>SYRSRSAFKLLEVNERHQILRPGLRVLDCGAAPGAWSQVAVQKVNAAGTDPSSPVGFVLGVDLLHIFPLEGATFLCPADVTDPRTSQRILEVLPGRRADVILSDMAPNATGFRDLDHDRLISLCLTLLSVTPDILQPGGTFLCKTWAGSQSRRLQRRLTEEFQNVRIIKPEASRKESSEVYFLATQYHGRKGTVKQ[2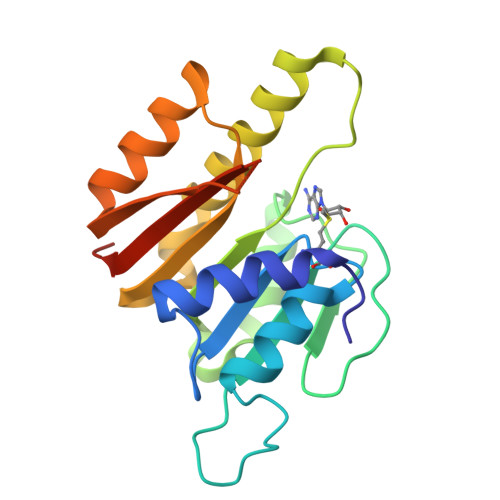x]> QHMEGNGPAAVHYQPASPPRDACVYSSCYS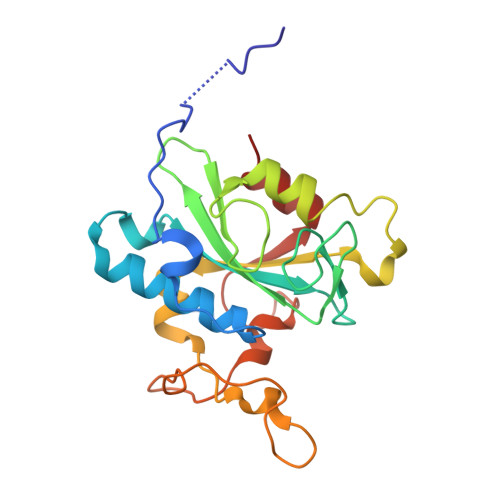EENVWKLCEYIKNHDQYPLEECYAVFISNERKMIPIWKQQARPGDGPVIWDYHVVLLHVSSGGQSFIYDLDTVLPFPCLFDTYVEDAIKSDDDIHPQFRRKFRVICADSYLKNFASDRSHMKDSSGNWREPPPPYPCIETGDSKMNLNDFISMDPKVGWGAVYTLSEFTHRFGS>[2x]MEKNFVITDPRLPDNPIIFASDGFLELTEYSREEILGRNARFLQGPETDQAT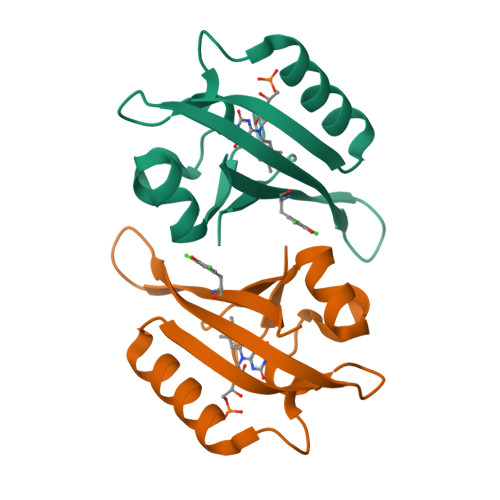VQKIRDAIRDQRETTVQLINYTKSGKKFWNLLHLQPVRDQKGELQYFXGVQLDGSDHVLEHHHHHH> GSHMASMRVLLAPMEGVLDSLVRELLTEVNDYDLCITEFVRVVDQLLPVKVFHRICPELQNASRTPSGTLVRVQLLGQFPQWLAENAARAVELGSWGVDLNCGAPSKTVNGSGGGATLLKDPELIYQGAKAMREAVPAHLPVSVKVRLGWDSGEKKFEIADAVQQAGATELVVHGRTKEQGYRAEHIDWQAIGDIRQRLNIPVIANGEIWDWQSAQQCMAISGCDAVMIGRGALNIPNLSRVVKYNEPRMPWPEVVALLQKYTRLEKQGDTGLYHVARIKQWLSYLRKEYDEATELF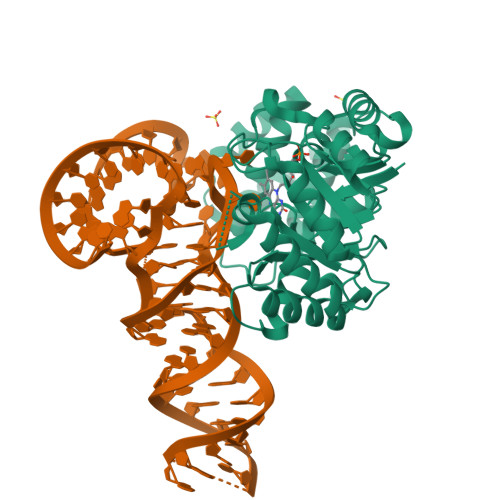QHVRVLNNSPDIARAIQAIDIEKL The COMMD (Copper Metabolism Murr1 (Mouse U2af1-rs1 region 1) Domain) proteins are highly conserved in metazoans and unicellular protozoa. There are ten family members that play key roles in intracellular trafficking and in the regulation of transcription. A hallmark of the COMMD family members is a highly conserved C-terminal sequence of ~70–80 amino acids called the COMM domain, which has no known structure. The N-terminal domain of these proteins, which we refer to as the HN (helical N-terminal) domain, is more variable in sequence across the ten proteins, and is proposed to ascribe unique functions to the different family members.

We next determined the structure of the Commd9 N-terminal domain by X-ray crystallography to a resolution of 1.55 Å using multi-wavelength anomalous dispersion. Overall, the Commd9 N-terminal domain has a globular architecture and is composed of a six-helix bundle with a meander topology. We therefore refer to this domain as the HN (Helical N-terminal) domain. The overall structure of the HN domain has a similar all α-helical fold to the equivalent domain of Commd1, which was previously determined by NMR. Compared to Commd1 however, the HN domain of Commd9 has an additional α-helix at its N-terminus that packs down on top of the structure, and a large disordered loop in Commd1 is better resolved in Commd9. In Commd9 the α4 helix forms a central core element that extends the length of the HN domain. However, the topology of the five shared α-helices (α2-α6) is similar overall. Comparing the HN domains of Commd1 and Commd9 using DALI showed structural similarity (DALI Z-score >3) with an RMSD of 3.2 Å over 83 Cα atoms. The electrostatic surface of the Commd9 HN domain reveals the presence of two basic patches and a negatively charged region, but it is not clear yet what their functional significance might be. Mapping sequence conservation of the Commd9 HN domain across species shows conserved surface residues mainly in the α1 helix region.

>[2x]MSGAMAALTAEHFAALQSLLKASSKDVVRQLCQESFSSSALGLKKLLDVTCSSLSVTQEEAEELLQALHRMTRLVAFRDLSSAEAILALFPENFHQNLKNLLTKIMLEHVSTWRTEAQANQ>[4x]MKRIGVLTSGGDSPGMNAAIRSVVRKAIYHGVEVYGVYHGYAGLIAGNIKKLEVGDVGDIIHRGGTILYTARCPEFKTEEGQKKGIEQLKKHGIEGLVVIGGDGSYQGAKKLTEHGFPCV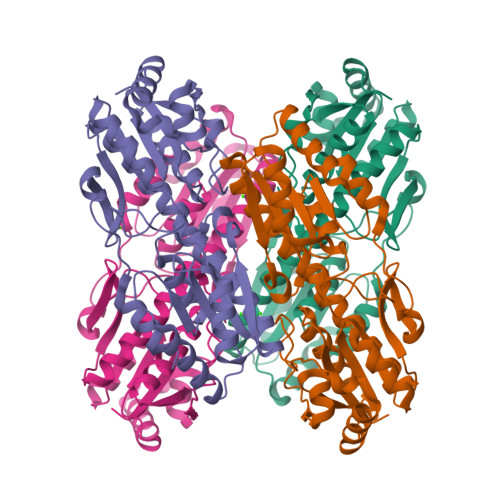GVPGTIDNDIPGTDFTIGFDTALNTVIDAIDKIRDTATSHERTYVIEVMGRHAGDIALWSGLAGGAETILIPEADYDMNDVIARLKRGHERGKKHSIIIVAEGVGSGVDFGRQIQEATGFETRVTVLGHVQRGGSPTAFDRVLASRLGARAVELLLEGKGGRCVGIQNNQLVDHDIAEALANKHTIDQRMYALSKELSI> MK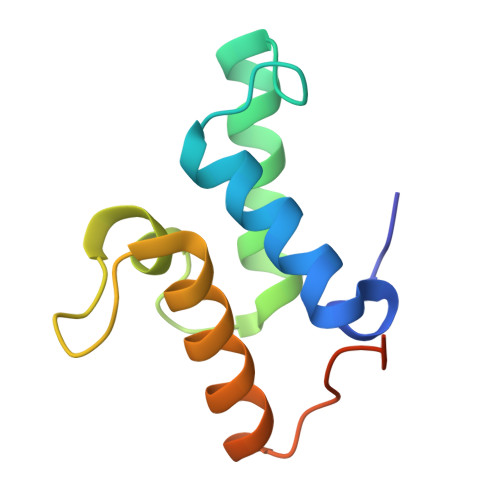SKISEYTEKEFLEFVKDIYTNNKKKFPTEESHIQAVLEFKKLTEHPSGSDLLYYPNENREDSPAGVVKEVKEWRASKGLPGFKAGLEHHHHHH2-(3-[3-({3-[(benzylamino)methyl]-4-chlorophenyl}ethynyl)-4-chlorophenyl]-1-{3-[(3S)-3-methylmorpholin-4-yl]propyl}-1,4,6,7-tetrahydro-5H-pyrazolo[4,3-c]pyridin-5-yl)-2-oxoacetamide 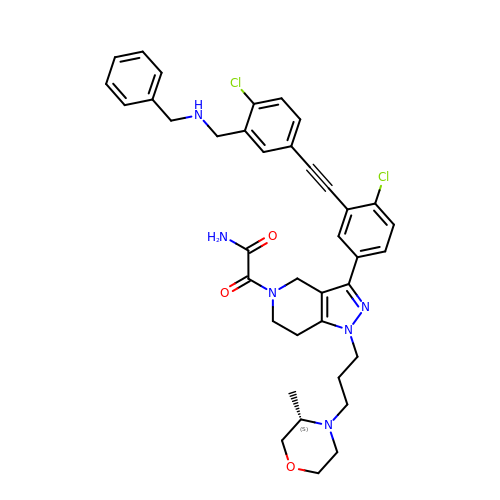| C38 H40 Cl2 N6 O3 | CIONECARUUEYBQ-SANMLTNESA-N1-{[7-(5-chloro-2-{[(3R,4S)-4-fluoropyrrolidin-3-yl]oxy}-3-methylphenyl)thieno[3,2-b]pyridin-2-yl]methyl}-1H-pyrrole-2,5-dione 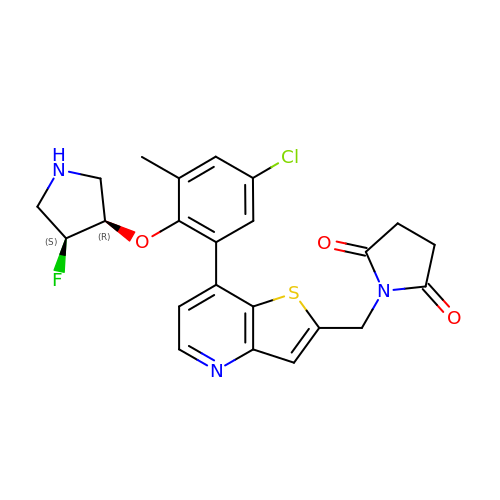| C23 H21 Cl F N3 O3 S | SWLBIOVQZDSJKD-PKOBYXMFSA-N> VNPGVVVRISQKGLDYASQQGTAALQKELKRIKIPDYSDSFKIKHLGKGHYSFYSMDIREFQLPSSQISMVPNVGLKFSISNANI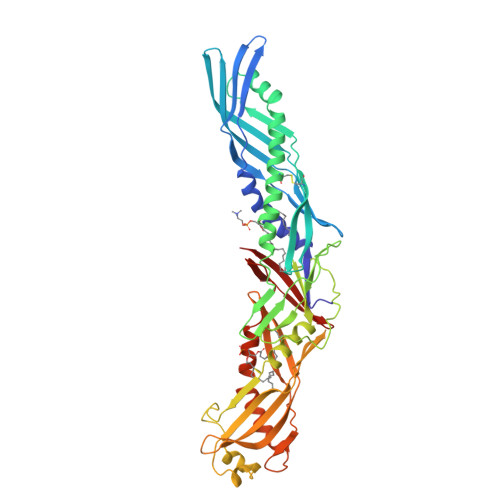KISGKWKAQKRFLKMSGNFDLSIEGMSISADLKLGSNPTSGKPTITCSSCSSHINSVHVHISKSKVGWLIQLFHKKIESALRNKMNSQVCEKVTNSVSSKLQPYFQTLPVMTKIDSVAGINYGLVAPPATTAETLDVQMKGEFYSENHHNPPPFAPPVMEFPAAHDRMVYLGLSDYFFNTAGLVYQEAGVLKMTLRDDMIPKESKFRLTTKFFGTFLPEVAKKFPNMKIQIHVSASTPPHLSVQPTGLTFYPAVDVQAFAVLPNSALASLFLIGMHTTGSMEVSAESNRLVGELKLDRLLLELKHSNIGPFPVELLQDIMNYIVPILVLPRVNEKLQKGFPLPTPARVQLYNVVLQPHQNFLLFGADVVYK> MGHHHHHHSIETDRVSKEFIEFLKTFHKTGQEIYKQTKLFLEGMHYKRDLSIEEQSECAQDFYHNVAERMQTRGKVPPERVEKIMDQIEKYIMTRLYKYVFCPETTDDEKKDLAIQKRIRALRWVTPQMLCVPVNEDIPEVSDMVVKAITDIIEMDSKRVPRDKLACITKCSKHIFNAIKITKNEPASADDFLPTLIYIVLKGNPPRLQSNIQYITRFCNPSRLMTGEDGYYFTNLCCAVAFIEKLDAQSLNLSQEDFDRYMSQMYKNLDLLSQLNERQERIMNEAKKLEKDLIDWTDGIAREVQDIVEK;>METRDQVKKLQLMLRQANDQLEKTMKDKQELEDFIKQSSEDSSHQISALVLRAQASEILLEELQQGLSQAKRDVQEQMAVLMQSREQVSEEL[2x]

In this process, small GTPase Rab5 functions as a master regulator of the early endosomal biogenesis. Rabex-5 is a specific GEF for Rab5, Rab17, and Rab21. Rabaptin-5 is a key effector of Rab5 and plays an important role in both homotypic and heterotypic fusions of early endosomes. The GEF activity of Rabex-5 is autoinhibited by its CC domain and is activated by the binding of Rabaptin-5 via its C2-1 domain.

In the R2Δ complex, the linker between the Rabex-5 GEF and CC domains was removed to facilitate the crystallization. On the other hand, in the structure of the R2Δ complex, Rabaptin-5C212 forms 2 two-helix bundles with a V-shaped conformation, and Rabex-5CC interacts via the nonpolar surface with the C-terminal regions of Rabaptin-5C212 to form a tight three-helix bundle. Rabex-5CC (residues 413–452) forms a long amphipathic α-helix (about 60 Å) that is in agreement with the prediction by Delprato and Lambright (2007). It packs in parallel with the C-terminal α-helices of Rabaptin-5C212 to form a tight three-helix bundle with its nonpolar surface buried in a hydrophobic surface groove of Rabaptin-5C212. The interactions are dominantly hydrophobic that bury a total of solvent accessible surface area of 2664 Å2. The GEF domain packs along the three-helix bundle formed by Rabex-5CC and Rabaptin-5C212. The interaction interface buries a total of solvent accessible surface area of 1040 Å2, which is much smaller than that between Rabex-5 and Rab21 (2400 Å2). Hence, we consider that the substrate-binding site of Rabex-5 is largely exposed to the solvent and partially accessible by the substrate. In the structure of the R2Δ complex, the substrate-binding site of Rabex-5 is partially occupied by Rabex-5CC and Rabaptin-5C212, implying that further conformational change(s) of the R2Δ complex will be required to bind Rab5. The not-so-tight interaction of the Rabex-5 GEF domain with Rabex-5CC and Rabaptin-5C212 as observed in the R2Δ structure allows the conformational changes easily during the substrate binding.>KPGKATGKGKPVNNKWLNNAGKDLGSPVPDRIANKLRDKEFKSFDDFRKKFWEEVSKDPELSKQFSRNNNDRMKVGKAPKTRTQDVSGKRTSFE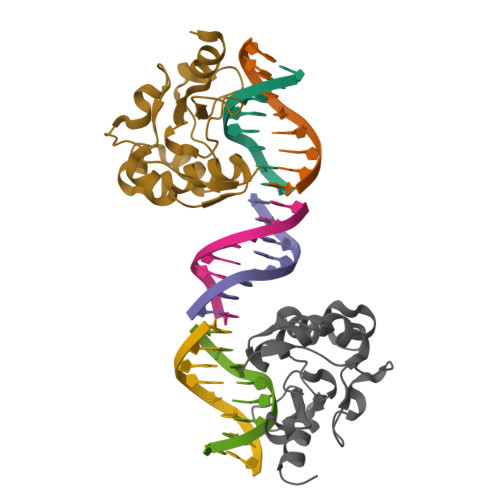LHHEKPISQNGGVYDMDNISVVTPKRHIDIHRGK[2x]>MGDSMISSATSDTGSAKRKSKKNIRKQRMKILFNVVLEAREPGSGRRLCDLFMVKPSKKDYPDYYKIILEPMDLKIIEHNIRNDKYAGEEGMIEDMKLMFRNARHYNEEGSQVYNDAHILEKLLKEKRKELGPLPDDDDMASPA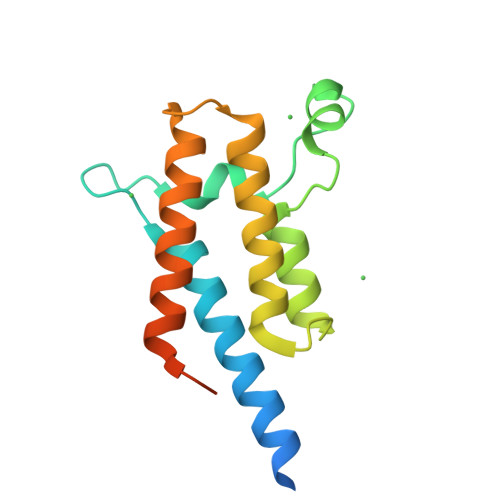ENLYFQ[2x]>[2x]MASSSTPRFRVYSKYLFLTYPQCTLEPQYALDSLRTLLNKYEPLYIAAVRELHEDGSPHLHVLVQNKLRASITNPNALNLRMDTSPFSIFHPNIQAAKDCNQVRDFITKEVDSDVNTAEWGTFVAVSTPGRKDRDADLE

Replication initiator proteins (Reps) from the HUH-endonuclease superfamily process specific single-stranded DNA (ssDNA) sequences to initiate rolling circle/hairpin replication in viruses, such as crop ravaging geminiviruses and human disease causing parvoviruses. At the heart of DNA processing of all HUH-endonucleases is a structurally defined catalytic nickase domain that first recognizes a specific sequence/structure of DNA; nicks ssDNA at a ‘nic site’ to yield a sequestered 5′ end that remains covalently bound to the HUH endonuclease and a free 3′OH that can be used as a primer for DNA replication; and finally, facilitates a strand transfer reaction to resolve the covalent intermediate. To uncover the ssDNA recognition mechanism of Reps and identify potential motifs that might confer sequence specificity, we solved the first high resolution crystal structures of two Rep nickase domains from Porcine circovirus 2 (PCV2) and Wheat dwarf virus (WDV) with 12% sequence identity, bound to ssDNA encoding minimal sequences comprising the respective origin of replication (ori) sequences. With this, we term this turn-β-turn structural motif as the ‘single-stranded DNA Bridging Motif’ (sDBM), and suggest that it is the main binding moiety responsible for recognition and conformation priming of ssDNA by Rep HUH-endonucleases.

We present structures of two 10-mer bound structures of inactive PCV2Y96F (1.93 Å resolution) and WDVY106F (1.80 Å resolution), and one 8-mer bound WDVY106F (2.61 Å resolution) structure. The pre-cleavage state was captured by mutating the catalytic tyrosine to phenylalanine. All three structures are in complex with the divalent cofactor manganese. Strikingly, despite the absence of bases that make up the hairpin stem in the short target DNA oligos, the ssDNA is bent into a ‘U-shaped’ architecture like one might expect in the context of the hairpin loop. A comprehensive table containing BASA and contact values of each of the three structures featured in this study is also provided.> MFVATSLLLAIATLVVRASPHNYLIMDIEPPKSVSERDILNLLSPLQVKHSFRVTGSTRLLIVIRLDAQSYEKLDEITVPGKVEVIPAVNMADTMERCGVSWPRVELTDDNVTLFESESTLTDVTKEQLKAMLIGYGEHMSGLLQAHRFEYYQAAGATPHRHFVFVNSVPDE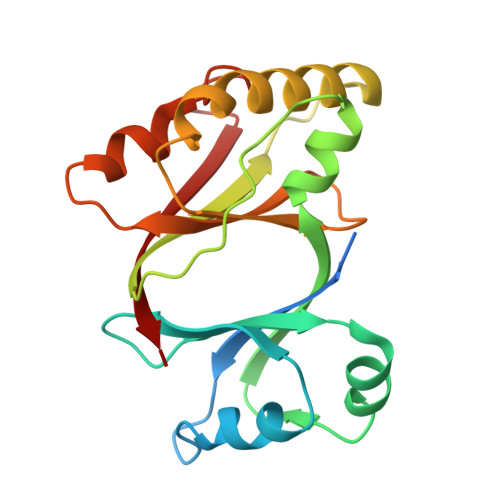IEVFGREGVDIWGGPGEFVVKPQYVTRI> MSNLNLFATILTYPAPASNYRGESEENRSVIQKILKDGQKYAIISPESMRNALREMLIELGQPNNRTRLHSEDQLAVEFKEYPNPDKFADDFLFGYMVAQTNDAKEMKKLNRPAKRDSIFRCNMAVAVNPYK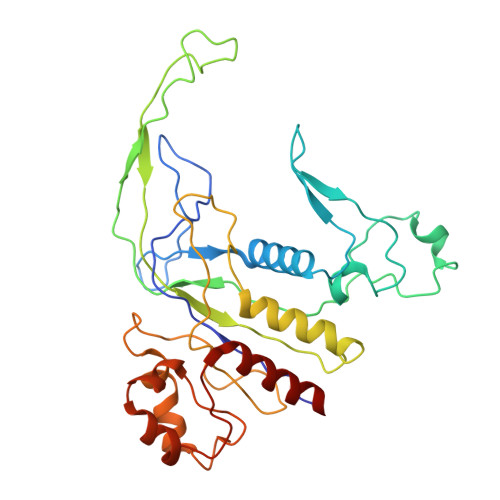YDTVFYQSPLNAGDSAWKNSTSSALLHREVTHTAFQYPFALAGKDCAAKPEWVKALLQAIAELNGVAGGHARAYYEFAPRSVVARLTPKLVAGYQTYGFDAEGNWLELSRLTATDSDNLDLPANEFWLGGELVRKMDQEQKAQLEAMGAHLYANPEKLFADLADSFLGV> GSTMSLSRSEEMHRLTENVYKTIMEQFNPSLRNFIAMGKNYEKALAGVTYAAKGYFDALVKMGELASESQGSKELGDVLFQMAEVHRQIQNQLEEMLKSFHNELLTQLEQKVELDSRYLSAALKKYQTE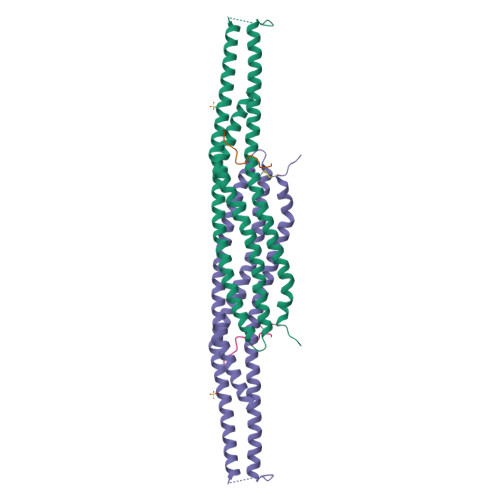QRSKGDALDKCQAELKKLRKKSQGSKNPQKYSDKELQYIDAISNKQGELENYVSDGYKTALTEERRRFCFLVEKQCAVAKNSAAYHSKGKELLAQKLPLWQQACADPSKIPERAVQLMQQVASN;> GTVQNPYADVKTX>ATCATAWSSSSVYTNGGTVSYNGRNYTAKWWTQNERPGTSDVWADKGACGTGGEGPGGNNGFVVSEAQFNQMFPNRNAFYTYKGLTDALSAYPAFAKTGSDEVKKREAAAFLANVSHETGGLFYIKEVNEANYPHYCDTTQSYGCPAGQAAYYGRGPIQLSWNFNYKAAGDALGINLL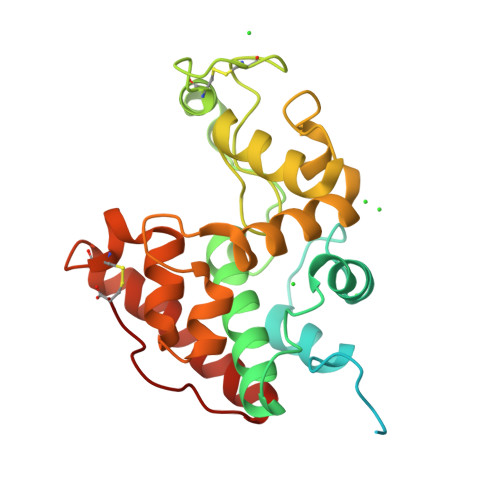ANPYLVEQDPAVAWKTGLWYWNSQNGPGTMTPHNAIVNNAGFGETIRSINGALECNGGNPAQVQSRINKFTQFTQILGTTTGPNLSC[2x]>[2x]GPLGSMSGGFELQPRDGGPRVALAPGETVIGRGPLLGITDKRVSRRHAILEVAGGQLRIKPIHTNPCFYQSSEKSQLLPLKPNLWCYLNPGDSFSMLVDKYIFRILSIPSA;>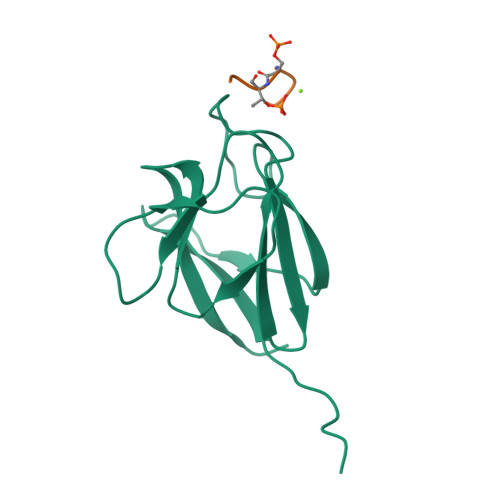AYDESTDEE[2x]> DSKLSIISWNVDGLDTLNLADRARGLCSYLALYTPDVVFLQELIPAYVQYLKKRAV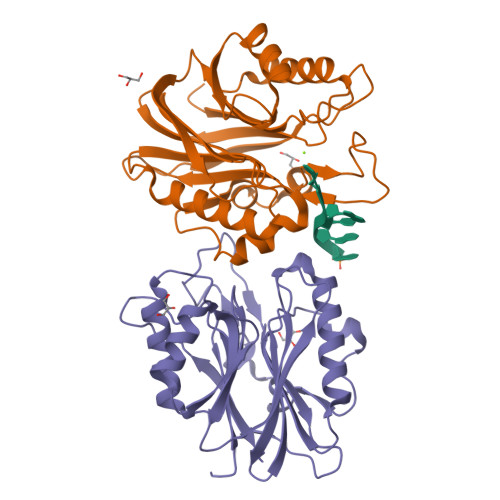SYLFFEGSDDGYFTGIMLRKSRVKFLESEIICFPTTQMMRNLLIAQVTFSGQKLYLMTSHLESCKNQSQERTKQLRVVLQKIKEAPEDAIVIFAGDTNLRDAEVANVGGLPAGVCDVWEQLGKQEHCRYTWDTKANSNKTVPYVSRCRFDRIFLRSAKTAPPVTPDHMALIGMEKLDCGRYTSDHWGIYCTFNT;> EDSKLSIISWNVDGLDTLNLADRARGLCSYLALYTPDVVFLQELIPAYVQYLKKRAVSYLFFEGSDDGYFTGIMLRKSRVKFLESEIICFPTTQMMRNLLIAQVTFSGQKLYLMTSHLESCKNQSQERTKQLRVVLQKIKEAPEDAIVIFAGDTNLRDAEVANVGGLPAGVCDVWEQLGKQEHCRYTWDTKANSNKTVPYVSRCRFDRIFLRSAKTAPPVTPDHMALIGMEKLDCGRYTSDHWGIYCTFNT RepB, the replication initiation protein of pMV158, is a member of the HUH endonuclease superfamily, which includes proteins involved in the replication of plasmids, bacteriophages and viruses, as well as proteins with roles in DNA transposition and in conjugative mobilisation of plasmids. These proteins are characterised by the presence of two conserved protein motifs: the HUH motif, composed of two His residues separated by a bulky hydrophobic amino acid, which is responsible for the coordination of a divalent metal cation, and the catalytic motif, containing one or two Tyr residues separated by several amino acids. Each monomer of RepB comprises two domains connected by a short hinge region. The C-terminal or oligomerisation domain (OD) is a helical domain responsible for the hexameric state of the protein, while the N-terminal or origin binding domain (OBD) carries the catalytic active site and is in charge of recognising, cleaving and joining dso DNA.

The OBD was crystallised in complex with a 23-bp dsDNA fragment (23AB) containing two out of the three repeats from the bind locus. In this complex, the asymmetric unit consisted of two molecules of the DNA oriented in opposite directions, and two molecules of OBD bound to each DNA molecule. The DNA molecules are in B conformation, with an estimated curvature of the DNA of ∼25°. The two OBDs are positioned on the same side of the DNA molecule because they are all bound to the GC-rich region within the 11-bp tandem direct repeats, which are separated by a complete double helix turn. The binding to the GC-rich region in the absence of DNA bending causes the lack of protein-protein interactions between the OBDs bound on the same DNA molecule, in agreement with our results indicating that there was no cooperative binding of the OBD to the DNA (see above). The binding of the OBD to the DDR drives this latter loop to move 3.16 Å away so that Met86 locates at approximately 3.0 Å of G8 of the top strand in the OBD–DDR structure. This movement includes the 180° flip of the Ala85-Met86 peptide bond and results in the extension of strand β4 by four residues in the N-term direction. The interaction of the OBD with the DNA of the bind locus occurs through the major groove and involves residues situated in the N-terminal part of the domain, namely the N-terminal tail, the α2 helix, and the neighbouring loops connecting to β3, α2 and β4, and the extended strand β4 or anchoring strand. More extensive are the contacts of the α2 helix, which fully penetrates the major groove, adjacent to where the N-terminal tail is situated. Regarding the structure of the OBD bound to DNA, it is noteworthy that in the OBD–DDR complex, the active site is not found in the vicinity of the DNA.

>MKHHHHHHQAKEKARYFTFLLYPESIPSDWELKLETLGVPMAISPLHDKDKSSIKGQKYKKAHYHVLYIAKNPVTADSVRKKIKLLLGEKSLAMVQVVLNVENMYLYLTHESKDAIAKKKHVYDKADIKLINNFDIDRYV[4x]> MANRTVSPSTQGVRPAMRQMYNGRNVAT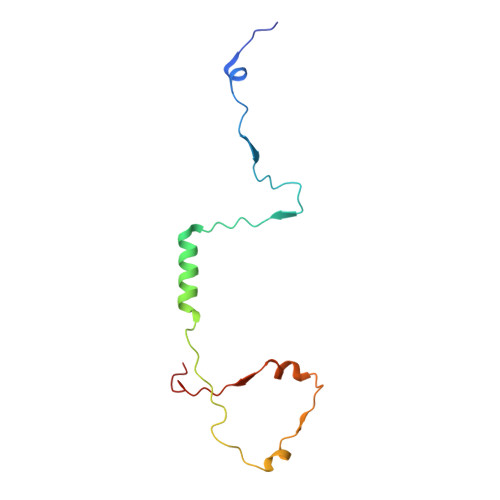RPIPLIVDTSEIRAIMAAAADARPKTSAVNFPQSGPRPAGAAVVFGTKVSGAPGNVVSNNAATFAPLTGTQNFE> NTGLLESQLSRHDQMLSVHDIRLADMDLRFQVLETASYNGVLIWKIRDYKRRKQEAVMGKTLSLYSQPFYTGYFGYKMCARVY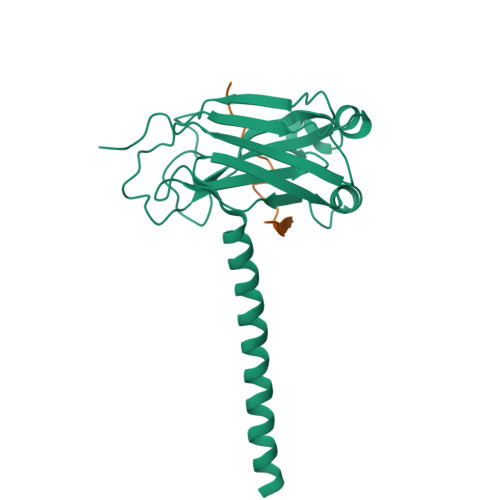LNGDGMGKGTHLSLFFVIMRGEYDALLPWPFKQKVTLMLMDQGSSRRHLGDAFKPDPNSSSFKKPTGEMNIASGCPVFVAQTVLENGTYIKDDTIFIKVIVDTSDLPDP;> SVPIQCTDKTDKQEALFK>MTGSEIFLASKRAAITYDTDPATGEPRAWLAPGGTGNVVAEQAGVLNISWIASADSEDDRRASALNPDGVTMELHSGREILVRLIRHDPAVFRNVQNFMTANLMWAANNYGWDRWTQPSFGSDAREGWADFGRFTRDFADAILKSSAQSADPVYLVHDYQLVGVPALLREQRPDAPILLFVHIPWPSADYWRILPKEIRTGILHGMLPATTIGFFADRWCRNFLESVADLLPDARIDREAMTVEWRGHRTRLRTMPLGYSPLTLDGRNPQLPEGIEEWADGHRLVVHSGRTDPIKNAERAVRAFVLAARGGGLEKTRMLVRMNPNRLYVPANADYVHRVETAVAEANAELGSDTVRIDNDNDVNHTIACFRRADLLIFNSTVDGQNLSTFEAPLVNERDADVILSETCGAAEVLGEYCRSVNPFDLVEQAEAISAALAAGPRQRAEAAARRRDAARPWTLEAWVQAQLDGLAADHAARTATAERFDTAPAVSTRADL[6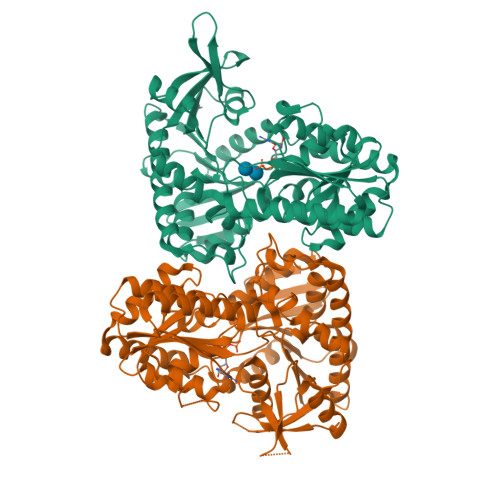x]> MKLAILGAGCYRTHAASGITNFSRACEVAEMVGKPEIAMTHSTITMGAELKELAGVDEVVVADPVFDNQFTVIDDFAYEDVIEAHKEDPEKIMPQIREKVNEVAKELPKPPEGAIHFTHPEDLGFEITTDDREAVADADFIMTWFPKGDMQPDIINKFIDD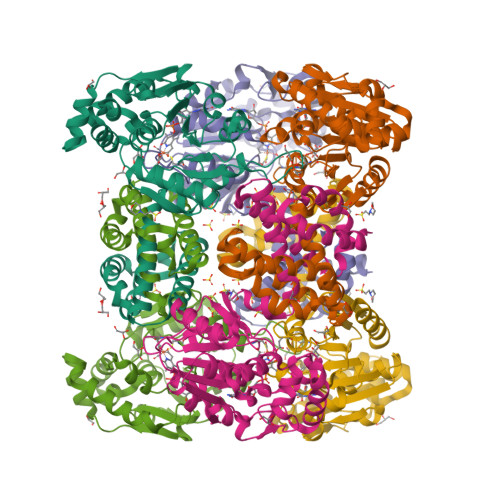IKPGAIVTHACTIPTTKFYKIFEQKHGDLVTKPETLNVTSYHPGAVPEMKGQVYIAEGYASEDAIETLFELGQKARGNAYRLPAELLGPVCDMCSALTAITYAGILSYRDSVTQVLGAPASFAQMMAKESLEQITALMEKVGIDKMEENLDPGALLGTADSMNFGASAEILPTVFEILEKRKK(2R,4S)-2-[(1R)-1-{[(6S)-6-carboxy-6-(glycylamino)hexanoyl]amino}-2-oxoethyl]-5,5-dimethyl-1,3-thiazolidine-4-carboxylic acid | C17 H28 N4 O7 S | 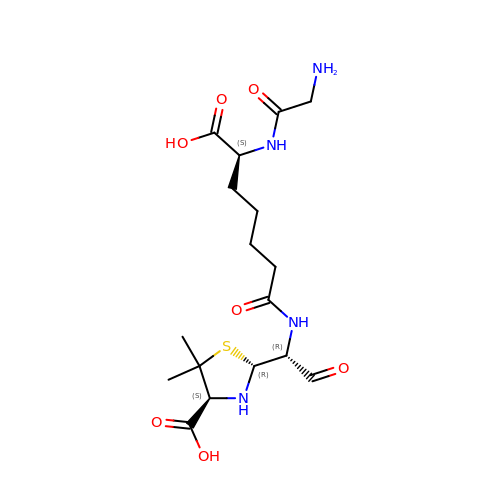GWAZTQMEPPXKKK-GIFSMMMISA-N>[2x]QKEGVLRVITRNSPATYFQDRNGETGFEYELAKRFAERLGVELKIETADNLDDLYAQLSREGGPALAAAGLTPGREDDASVRYSHTYLDVTPQIIYRNGQQRPTRPEDLVGKRIMVLKGSSHAEQLAELKKQYPELKYEESDAVEVVDLLRMVDVGDIDLTLVDSNELAMNQVYFPNVRVAFDFGEARGLAWALPGGDDDSLMN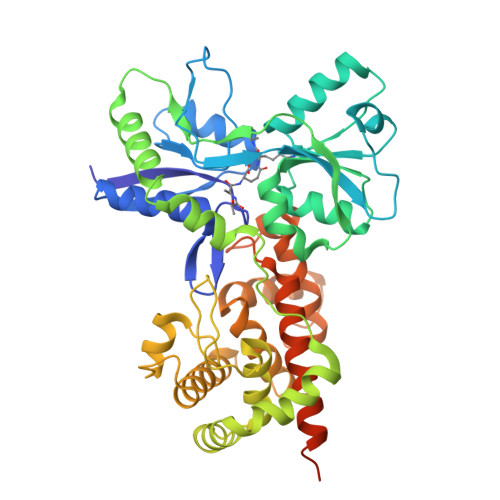EVNAFLDQAKKEGLLQRLKDRYYGHVDVLGYVGAYTFAQHLQQRLPRYESHFKQSGKQKDTDWRLLAAIGYQESLWQPGATSKTGVRGLMMLTNRTAQAMGVSNRLDPKQSIQGGSKYFVQIRSELPESIKEPDRSWFALAAYNIGGAHLEDARKMAEKEGLNPNKWLDVKKMLPRLAQKQWYAKTRYGYARGGETVHFVQNVRRYYDILTWVTQPQMEGSQIAESGLHLPGVNKTRPEEDSGDEKL;>[2x]QKEGVLRVITRNSPATYFQDRNGETGFEYELAKRFAERLGVELKIETADNLDDLYAQLSREGGPALAAAGLTPGREDDASVRYSHTYLDVTPQIIYRNGQQRPTRPEDLVGKRIMVLKGSSHAEQLAELKKQYPELKYEESDAVEVVDLLRMVDVGDIDLTLVDSNELAMNQVYFPNVRVAFDFGEARGLAWALPGGDDDSLMNEVNAFLDQAKKEGLLQRLKDRYYGHVDVLGYVGAYTFTQHLQQRLPRYESHFKQSGKQKDTDWRLLAAIGYQESLWQPGATSKTGVRGLMMLTNRTAQAMGVSNRLDPKQSIQGGSKYFVQIRSELPESIKEPDRSWFALAAYNIGGAHLEDARKMAEKEGLNPNKWLDVKKMLPRLAQKQWYAKTRYGYARGGETVHFVQNVRRYYDILTWVTQPQMEGSQIAESGLHLPGVNKTRPEEDSGDEKL> LKKQYIFQLSSLNPQERIDYCHLIEKLGGLVIEKQCFDPTCTHIVVGHPLRNEKYLASVAAGKWVLHRSYLEACRTAGHFVQEEDYEWGSSSILD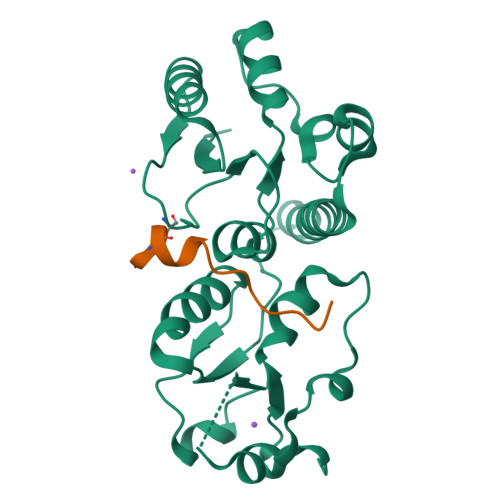VLTGINVQQRRLALAAMRWRKKIQQRQESGIVEGAFSGWKVILHVDQSREAGFKRLLQSGGAKVLPGHSVPLFKEATHLFSDLNKLKPDDSGVNIAEAAAQNVYCLRTEYIADYLMQESPPHVENYCLPEAISFI;> GACFKDAEYIYPSLESDDDDPA>GSAMARKRIITPEKKELIRNLISEYNITSAKDLQEALKDLLGDTIQNMLEAELDEHLGYEKYESTEEAKSNYRNGYTSKTLKSSVGQVEIDIPRDRNAEFEPKIVPRYKRDISEIENKIIAMYARGMSTREINEQIQEIYGFEVSAEMVSKITDKILPEIEEWQKRPLGEVYPIVFIDAIHFSVKNDGIVGKKAVYIVLAIDIEGQKDVIGIYVGENESSKFWLSVLNDLKNRGVKDILILCADALSGIKDAINAAFPNTEYQRCIVHQIRNTLKYVSDKDRKEFARDLKRIYTAPNEKAGYDQMLEVSEKWEKKYPAAMKSWKSNWDVICPFFKYSEELRKIMYTTNTIESLNSSYRRINKSRTVFPGDQSLLKSIYLATVKITSKWTMRYKNWGLILGQ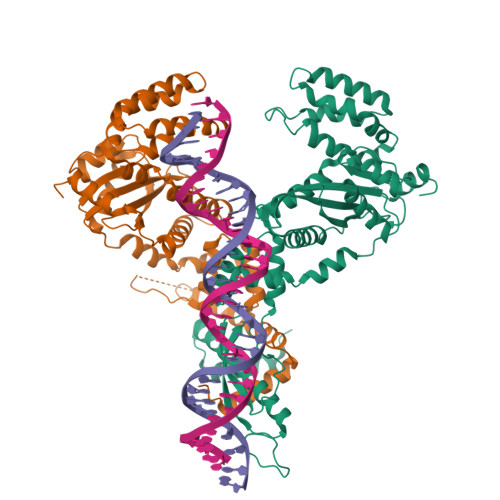LQIMFEGRI[2x]>[4x]WGQGTLVTVSAESARNPTIYPLTLPPALSSDPVIIGCLIHDYFPSGTMNVTWGKSGKDITTVNFPPALASGGRYTMSSQLTLPAVECPEGESVKCSVQHDSNPVQELDVNCSGPTP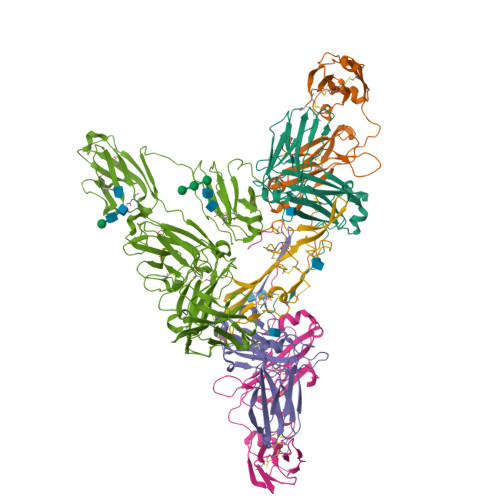PPPITIPSCQPSLSLQRPALEDLLLGSDASITCTLNGLRNPEGAVFTWEPSTGKDAVQKKAVQNSCGCYSVSSVLPGCAERWNSGASFKCTVTHPESGTLTGTIAKVTVNTFPPQVHLLPPPSEELALNELLSLTCLVRAFNPKEVLVRWLHGNEELSPESYLVFEPLKEPGEGATTYLVTSVLRVSAETWKQGDQYSCMVGHEALPMNFTQKTIDRLSGKPTNVSVSVIMSEGDGICY;> KSPIFGPQEVSSIEGDSVSITCYYPDTSVNRHTRKYWCRQGASGMCTTLISSNGYLSKEYSGRANLINFPENNTFVINIEQLTQDDTGSYKCGLGTSNRGLSFDVSLEVSQVPELPSDTHVYTKDIGRNVTIECPFKRENAPSKKSLCKKTNQSCELVIDSTEKVNPSYIGRAKLFMKGTDLTVFYVNISHLTHNDAGLYICQAGEGPSADKKNVDLQVLAPEPELLYKDLRSSVTFECDLGREVANEAKYLCRMNKETCDVIINTLGKRDPDFEGRILITPKDDNGRFSVLITGLRKEDAGHYQCGAHSSGLPQEGWPIQTWQLFVNEESTIPNRRSVVKGVTGGSVAIACPYNPKESSSLKYWCRWEGDGNGHCPVLVGTQAQVQEEYEGRLALFDQPGNGTYTVILNQLTTEDAGFYWCLTNGDSRWRTTIELQVAEATREPNLEVTPQNATAVLGETFTVSCHYPCKFYSQEKYWCKWSNKGCHILPSHDEGARQSSVSCDQSSQLVSMTLNPVSKEDEGWYWCGVKQGQTYGETTAIYIAVEER;> DDEATILADNKCMCTRVTSRIIPSTEDPNEDIVERNIRIVVPLNNRENISDPTSPLRRNFVYHLSDVCKKCDPVEVELEDQVVTATQSNICNEDDGVPETCYMYDRNKCYTTMVPLRYHGETKMVQAALTPDSCYPD>[3x]MTLWEDEMLDRMKGGFAATALLCLGLANPLAADTRTLSQQYLDDVRSGAIVIEGDSAAVSELILKRDIPIPYSYIAQLFATPNA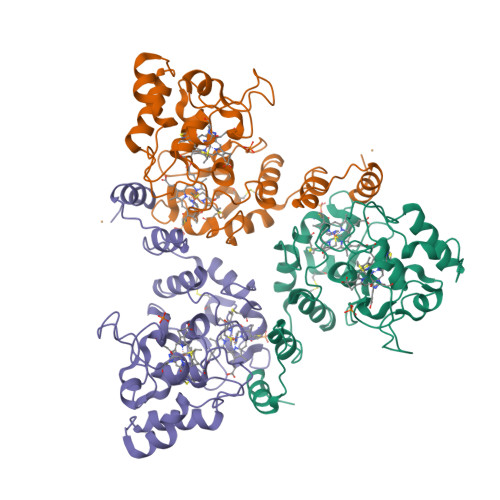FGSGPACIICHGSNNPTHAYRGLNLSTCDGLRNGSTEQPARAIFTPGEDPKNAIIGRRLRANRMPLGIAFNNPTDSAPILAIKEWILAGAPNDEHFTKEILPLFATDNTFGPDTPHCTTCHFSNQEPPSFHELNLTTYEGIMLGADSVAKGVDNATKVIIPGDPEASKVFQHLTEDRMPPGIDPSEDRDHPNTQILFAWIKQGAKCE pmcPolo-like kinase 1 (Plk1) is a mitotic serine/threonine (S/T) kinase, whose overexpression is closely associated with aggressiveness and poor prognosis for a wide spectrum of human cancers. Plk1 contains the C-terminal noncatalytic, but functionally essential, polo-box domain (PBD), which mediates interactions with its binding partners or substrates localized abundantly at centrosomes, kinetochores, and midbodies. Subsequent studies demonstrated that PBD serves as a structurally distinct protein–protein interaction (PPI) module for binding a short phospho-S/T (i.e., p-S/T)-containing motif. The polo-box domain (PBD), which serves as the substrate-recognition domain, is an attractive target for Plk1-specific anticancer drug discovery.

To characterize the binding mode of Allopole-A to PBD1, we determined the cocrystal structure of the PBD1•Allopole-A complex at 1.65 Å resolution. Analysis of the obtained structure showed that the two aromatic residues, W410 and F559, located 12.5 Å (Cα-Cα distance) away from each other, were critically required for Allopole-A binding. Interestingly, upon Allopole-A binding, the F559 phenyl ring present in multiple conformational isomers (Left) oriented itself parallel to the W410 indole ring to establish a π–π interaction with the heterocyclic aromatic ring of Allopole-A (Right). The indole ring of the W410 also tilted more than 20° to form another layer of the π–π interaction with the heterocyclic aromatic ring of Allopole-A (Inset). The W410 and F559 residues were surrounded by multiple hydrophobic residues (namely, I406, P407, I542, and I553), thus forming a water-shunning deep pocket (referred to hereafter as the W-F pocket). Moreover, P407 carbonyl established an H-bond with the Allopole-A triazole ring. Analysis with overlaid crystal structures showed that the L2 loop recruited to a phospholigand-bound PBD1 traverses over the W-F pocket and is not compatible with the Allopole binding to the pocket. Unsurprisingly, binding of Allopole-A to the W-F pocket displaced the L2 loop by sterically inhibiting the I497 binding to the W-F pocket and altering the hydrogen (H)- bonding capability of W410 and P407 with L2 loop backbone atoms. As a consequence, the intermolecular H-bond network of the L2 loop was not able to form and organize the ordered water-mediated interactions between the loop and a phospholigand. Thus, Allopole-A antagonizes the PBD1-dependent interaction with its phospholigands by “unstrapping” the L2 loop critical for securing a bound target.

> GAHMDCHLSDMLQQLHSVNASKPSERGLVRQEEAEDPACIPIFWVSKWVDYSDKYGLGYQLCDNSVGVLFNDSTRLILYNDGDSLQYIERDGTESYLTVSSHPNSLMKKITLLKYFRNYMSEHLLKAGANITPREGDELARLPYLRTWFRTRSAIILHLSNGSVQINFFQDHTKLILCPLMAAVTYIDEKRDFRTYRLSLLEEYGCCKELASRLRYARTMVDKLLSSR> MSEEKSRNGPARLKLVLGGATLGVVALATVAFGMKYTDQRPFCTSCHIMNPVGVTHKLSGHANISCNDCHAPHNLLA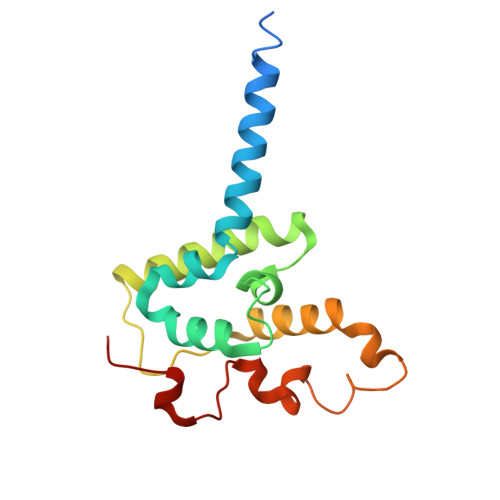KLPFKAIAGARDVYMNTLGHPGDLILAGMETKEVVNANCKACHTMTNVEVASMEAKKYCTDCHRNVQHMRMKPISTREVADE> GSHMASMTGGQQMGRGSMVKVLTACGNGMGSSMV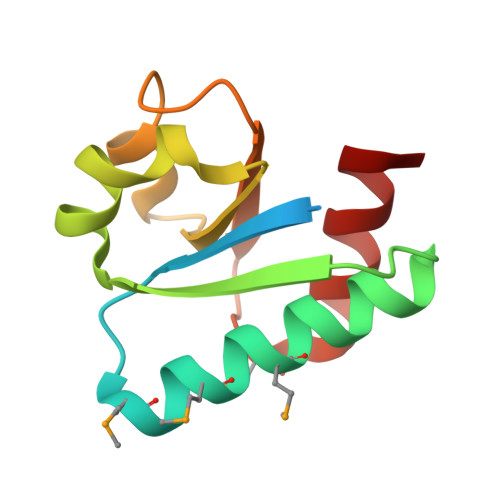IKMKVENALRQLGVSDIESASCSVGEAKGLASNYDIVVASNHLIHELDGRTNGKLIGLDNLMDDNEIKTKLEEALK>[4x]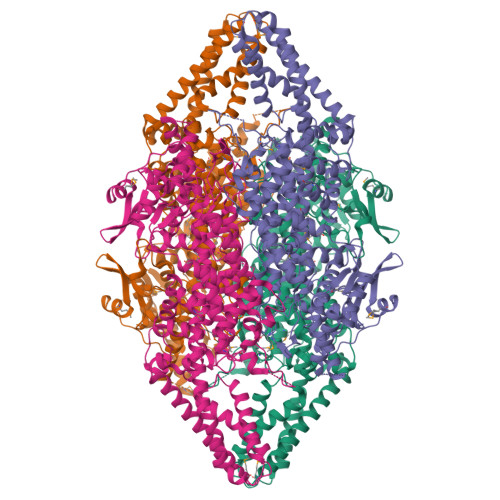MAPSLDSISHSFANGVASAKQAVNGASTNLAVAGSHLPTTQVTQVDIVEKMLAAPTDSTLELDGYSLNLGDVVSAARKGRPVRVKDSDEIRSKIDKSVEFLRSQLSMSVYGVTTGFGGSADTRTEDAISLQKALLEHQLCGVLPSSFDSFRLGRGLENSLPLEVVRGAMTIRVNSLTRGHSAVRLVVLEALTNFLNHGITPIVPLRGTISASGDLSPLSYIAAAISGHPDSKVHVVHEGKEKILYAREAMALFNLEPVVLGPKEGLGLVNGTAVSASMATLALHDAHMLSLLSQSLTAMTVEAMVGHAGSFHPFLHDVTRPHPTQIEVAGNIRKLLEGSRFAVHHEEEVKVKDDEGILRQDRYPLRTSPQWLGPLVSDLIHAHAVLTIEAGQSTTDNPLIDVENKTSHHGGNFQAAAVANTMEKTRLGLAQIGKLNFTQLTEMLNAGMNRGLPSCLAAEDPSLSYHCKGLDIAAAAYTSELGHLANPVTTHVQPAEMANQAVNSLALISARRTTESNDVLSLLLATHLYCVLQAIDLRAIEFEFKKQFGPAIVSLIDQHFGSAMTGSNLRDELVEKVNKTLAKRLEQTNSYDLVPRWHDAFSFAAGTVVEVLSSTSLSLAAVNAWKVAAAESAISLTRQVRETFWSAASTSSPALSYLSPRTQILYAFVREELGVKARRGDVFLGKQEVTIGSNVSKIYEAIKSGRINNVLLKMLA> APVL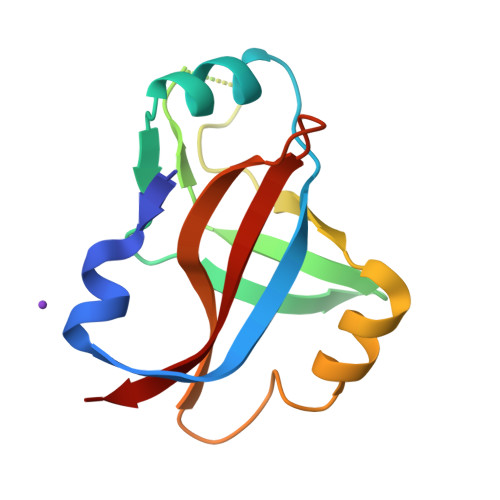ENRRARHDYEILETYEAGIALKGTEVKSLRAGKVDFTGSFARFEDGELYLENLYIAPYEKGSYANVDPRRKRKLLLHKHELRRLLGKVEQKGLTLVPLKIYFNERGYAKVLLGLARGK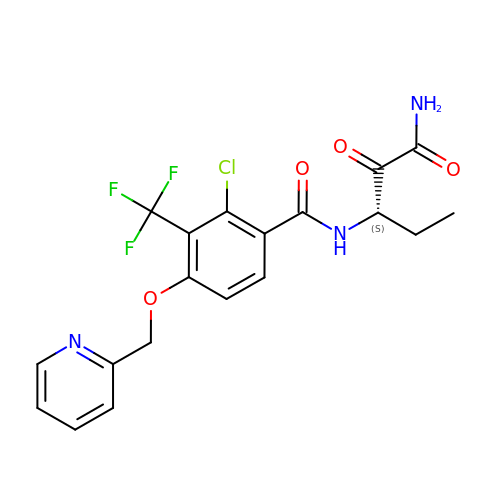N-[(1S)-3-amino-1-ethyl-2,3-dioxopropyl]-2-chloro-4-(pyridin-2-ylmethoxy)-3-(trifluoromethyl)benzamide | C19 H17 Cl F3 N3 O4 | VMSZYKRQEOLBRN-LBPRGKRZSA-N> MPGETITLQVGQCGNQVGLQYWQQLATEHGIQSDGSSTPYPKDINDLQLQELNNSGSSPQSYPQQTKPNGKYRNDHPELFFTLSDSNTYTPRSILI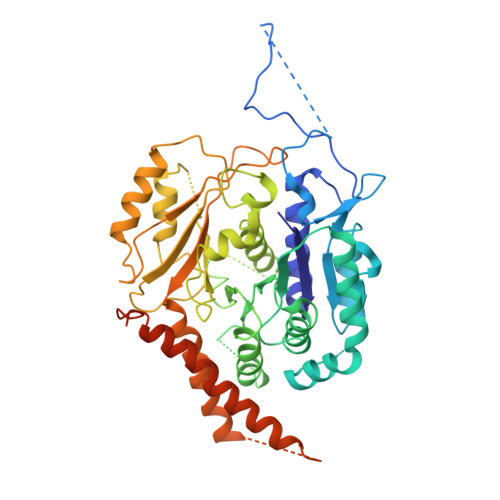DMEPSVIAKSTSALPMFNPRNVHLSNQGNGAANNWINGYKYGTEEEETLLNLIDREVDKCDNLSNFQLFHSVAGGTGSGVGSKMLEVISDRYGHKKLLNTFSIFPSNEDTSDVVVQPYNTILTLKRLIDYSDATFVFHNDSLNRIENILFNNNSNIQHDDNDLFLGANKLIALVSASVSNPLRFPGYMYSSMESIVSNLIPTPDLKFLTSSIAPFSTQKHNYLNEYDMLLELSNDRYKTNRVGGDTSYISMLNYLIGYNLDQREIRKGILKSQQRISFVPWVARSVLVVHGKKSPYLKNTNLEGIQVTNNTSMIDVFTKILKQFDLLIKRKAYLNRYYSSVEEENEVMEMFNESRESVKSIIDEYKACKEITYLDDDDEDDLEDGDGGGGGNGNGYNNIDDADMGI>MASTKAPGPGEKHHSIDAQLRQLVPGKVSEDDKLIEYDALLVDRFLNILQDLHGPSLREFVQECYEVSADYEGKGDTTKLGELGAKLTGLAPADAILVASSILHMLNLANLAEEVQIAHRRRNSKLKKGGFADEGSATTESDIEETLKRLVSEVGKSPEEVFEALKNQTVDLVFTAHPTQSARRSLLQKNARIRNCLTQLNAKDITDDDKQELDEALQREIQAAFRTDEIRRAQPTPQDEMRYGMSYIHETVWKGVPKFLRRVDTALKNIGINERLPYNVSLIRFSSWMGGDRDGNPRVTPEVTRDVCLLARMMAANLYIDQIEELMFELSMWRCNDELRVRAEELHSSSGSKVTKYYIEFWKQIPPNEPYRVILGHVRDKLYNTRERARHLLASGVSEISAESSFTSIEEFLEPLELCYKSLCDCGDKAIADGSLLDLLRQVFTFGLSLVKLDIRQESERHTDVIDAITTHLGIGSYREWSEDKRQEWLLSELRGKRPLLPPDLPQTEEIADVIGAFHVLAELPPDSFGPYIISMATAPSDVLAVELLQRECGVRQPLPVVPLFERLADLQSAPASVERLFSVDWYMDRIKGKQQVMVGYSDSGKDAGRLSAAWQLYRAQEEMAQVAKRYGVKLTLFHGRGGTVGRGGGPTHLAILSQPPDTINGSIRVTVQGEVIEFCFGEEHLCFQTLQRFTAATLEHGMHPPVSPKPEWRKLMDEMAVVATEEYRSVVVKEARFVEYFRSATPETEYGRMNIGSRPAKRRPGGGITTLRAIPWIFSWTQTRFHLPVWLGVGAAFKFAIDKDVRNFQVLKEMYNEWPFFRVTLDLLEMVFAKG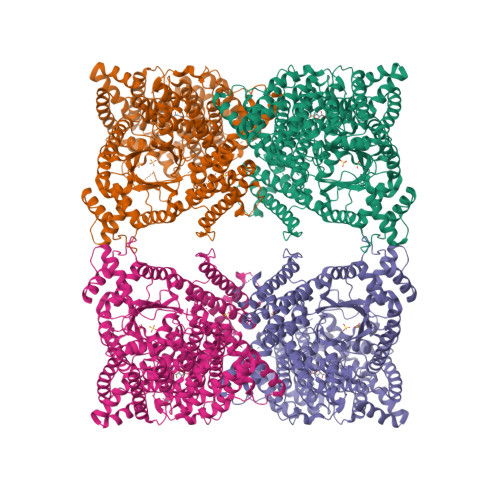DPGIAGLYDELLVAEELKPFGKQLRDKYVETQQLLLQIAGHKDILEGDPFLKQGLVLRNPYITTLNVFQAYTLKRIRDPNFKVTPQPPLSKEFADENKPAGLVKLNPASEYPPGLEDTLILTMKGIAAGMQNTG[4x]> GAMGSGAS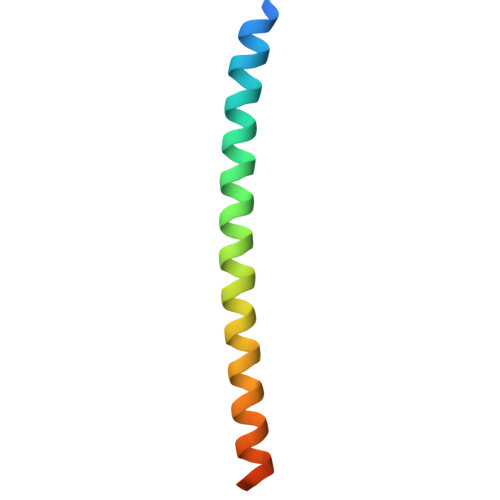SQAACLKQILLLQLDLIEQQQQQLQAKEKEIEELKSERDTLLARIERMERR butyl 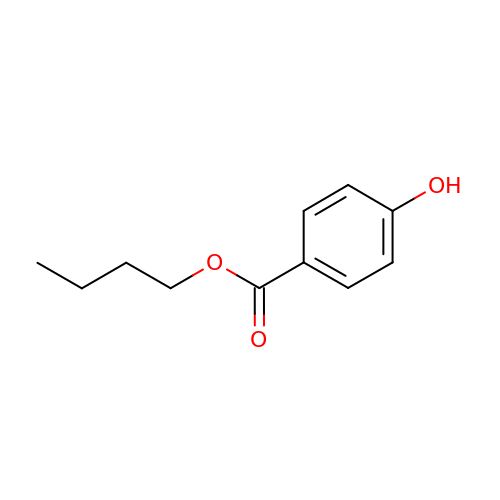4-hydroxybenzoate | C11 H14 O3 | QFOHBWFCKVYLES-UHFFFAOYSA-N>GGCAGGACUCGGCUUGCUGAAGC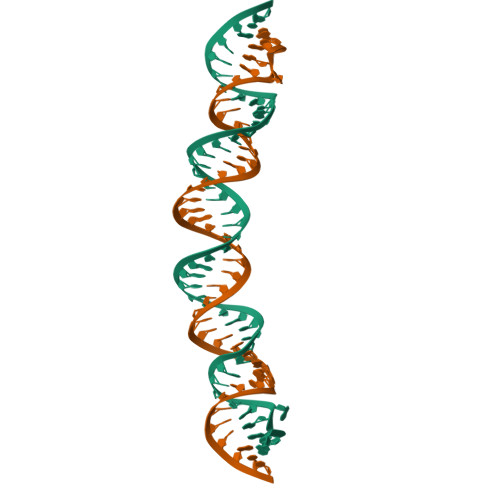GCGCACGGCAAGAGGCGAGGGGCC[2x]> MSTTVNVDSLAEYEKSQIKRALELGTVMTVFSFRKSTPERRTVQVIMETRQVAWSKTADKIEGFLDIMEIKEIRPGKNSKDFERAKAVRQKEDCCFTILYGTQFVLSTLSLAADSKEDAVNWLSGLKILHQEAMNASTPTIIESWLRKQIYSVDQTRRNSISLRELKTILPLINFKVSSAKFLKDKFVEIGAHKDELSFEQFHLFYKKLMFEQQKSILDEFKKDSSVFILGNTDRPDASAVYLHDFQRFLIHEQQEHWAQDLNKVRERMTKFIDDTMRETAEPFLFVDEFLTYLFSRENSIWDEKYDAVDMQDMNNPLSHYWISSSHNTYLTGDQLRSESSPEAYIRCLRMGCRCIELDCWDGPDGKPVIYHGWTRTTKIKFDDVVQAIKDHAFVTSSFPVILSIEEHCSVEQQRHMAKAFKEVFGDLLLTKPTEASADQLPSPSQLREKIIIKHKKLGPRGDVDVNMEDKKDEHKQQGELYMWDSIDQKWTRHYCAIADAKLSFSDDIEQTMEEEVPQDIPPTELHFGEKWFHKKVEKRTSAEKLLQEYCMETGGKDGTFLVRESETFPNDYTLSFWRSGRVQHCRIRSTMEGGTLKYYLTDNLTFSSIYALIQHYRETHLRCAEFELRLTDPVPNPNPHESKPWYYDSLSRGEAEDMLMRIPRDGAFLIRKREGSDSYAITFRARGKVKHCRINRDGRHFVLGTSAYFESLVELVSYYEKHSLYRKMRLRYPVTPELLERYNMERDINSLYDVSRMYVDPSEINPSMPQRTVKALYDYKAKRSDELSFCRGALIHNVSKEPGGWWKGDYGTRIQQYFPSNYVEDISTADFEELEKQIIEDNPLGSLCRGILDLNTYNVVKAPQGKNQKSFVFILEPKQQGDPPVEFATDRVEELFEWFQSIREITWKIDTKENNMKYWEKNQSIAIELSDLVVYCKPTSKTKDNLENPDFREIRSFVETKADSIIRQKPVDLLKYNQKGLTRVYPKGQRVDSSNYDPFRLWLCGSQMVALNFQTADKYMQMNHALFSLNGRTGYVLQPESMRTEKYDPMPPESQRKILMTLTVKVLGARHLPKLGRSIACPFVEVEICGAEYDNNKFKTTVVNDNGLSPIWAPTQEKVTFEIYDPNLAFLRFVVYEEDMFSDPNFLAHATYPIKAVKSGFRSVPLKNGYSED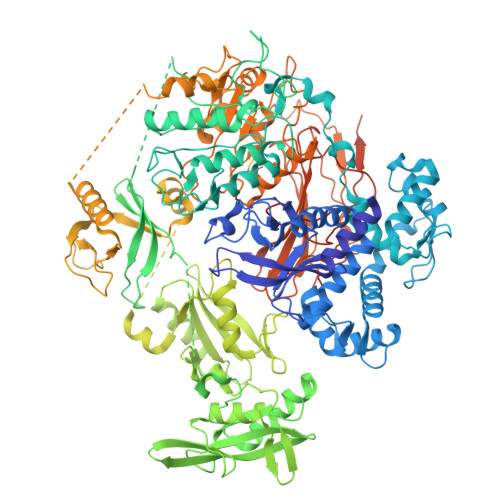IELASLLVFCEMRPVLESEEELYSSCRQLRRRQEELNNQLFLYDTHQNLRNANRDALVKEFSVNENQLQLYQEKCNKRLREKRVSNSKFYS> MPTKAVTFYEDINYGGASVSLQP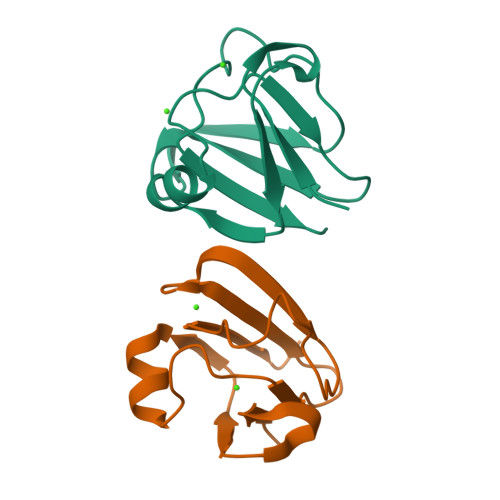GNYTLSQLNTAKIPNDDMTSLKVPSGWTVDVYENDNFTGTKWTYTSDTPWVGNDANDKMTSVKIYSTTNTGGDT>SNAAEHVRLATTTSTYHSGLLDYLLPQFEKDTGYKVDVIAAGTGKALKMGENGDVDLVMTHAPKAEGTFVEKGYGVLPRKLMYNDFVIVGPKADPAKIKDDESVLDVFKEIANKNATFISRGDDSGTHKKEMGFWAQTKIEPNFGGYRSVGQGMGPTLNMASEMQGYT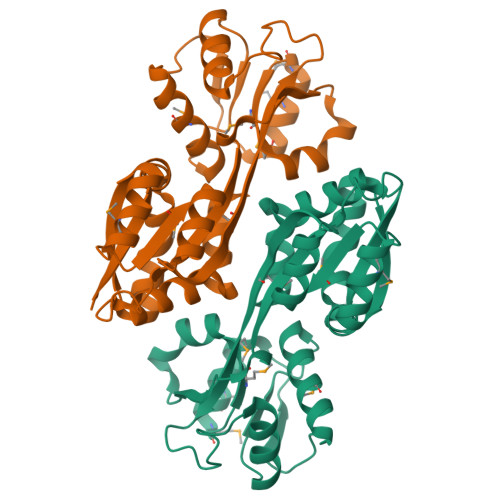MSDRGTWLAYQNKLDLEILFQGDEKLFNPYQVILVNPERYPTINYQGAKAFSDWLVNPRGQELINGFRL[2x]> MFSRPGLPVEYLQVPSASMGRDIKVQFQGGGPHAVYLLDGLRAQDDYNGWDINTPAFEEYYQSGLSVIMPVGGQSSFYTDWYQPSQSNGQNYTYKWETFLTREMPAWLQANKGVSPTGNAAVGLSMSGGSALILAAYYPQQFPYAASLSGFLNPSEGWWPTLIGLAMNDSGGYNAN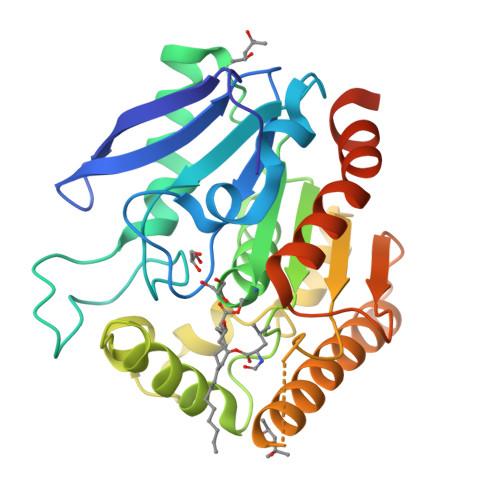SMWGPSSDPAWKRNDPMVQIPRLVANNTRIWVYCGNGTPSDLGGDNIPAKFLEGLTLRTNQTFRDTYAADGGRNGVFNFPPNGTHSWPYWNEQLVAMKADIQHVLNGATPPAAPAAPAALEHHHHHH> MAGRQAHRKFDVRNDTSTRWKGKLYGIFVNYMGEDYAKEFVEQAYSNYEKVFVNIYTKIHNQLRTTLTSSAGAGATFPLWQIINEAIYAVYLTHKETASFLYAKYVARGIQPNVVKKILAETGNALKGIVPAVAQELGETVLDESNVISVVDDIVRKNPALPNSYAGIILQEA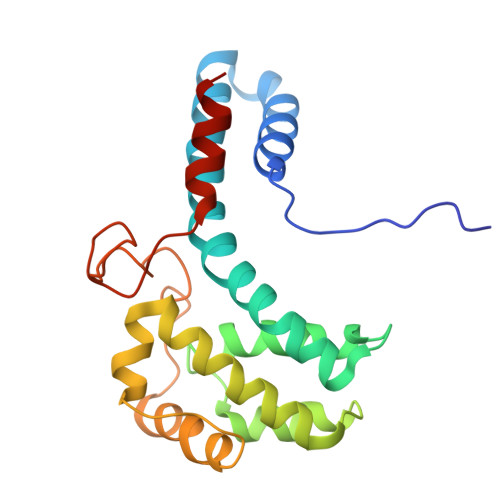RISTTPHYEGTEGFSSMESAYSALEEIEKGL>[4x]MQEKDASSQGFLPHFQHFAT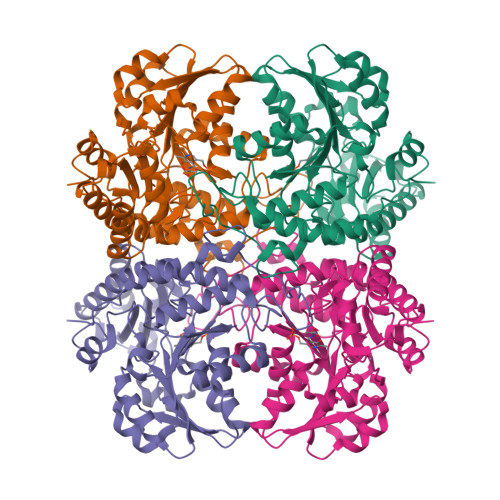QAIHVGQDPEQWTSRAVVPPISLSTTFKQGAPGQHSGFEYSRSGNPTRNCLEKAVAALDGAKYCLAFASGLAATVTITHLLKAGDQIICMDDVYGGTNRYFRQVASEFGLKISFVDCSKIKLLEAAITPETKLVWIETPTNPTQKVIDIEGCAHIVHKHGDIILVVDNTFMSPYFQRPLALGADISMYSATKYMNGHSDVVMGLVSVNCESLHNRLRFLQNSLGAVPSPIDCYLCNRGLKTLHVRMEKHFKNGMAVAQFLESNPWVEKVIYPGLPSHPQHELVKRQCTGCTGMVTFYIKGTLQHAEIFLKNLKLFTLAESLGGFESLAELPAIMTHASVLKNDRDVLGISDTLIRLSVGLEDEEDLLEDLDQALKAAHPPSG The most frequent PTM reaction catalyzed by FIC enzymes is the addition of AMP using ATP as a cofactor, coined AMPylation or adenylylation. Enterococcus faecalis FIC belongs to class III FIC proteins, which are comprised of a single FIC domain and carry an autoinhibitory glutamate in their C-terminal α-helix. We discover that EfFIC has both AMPylation and deAMPylation activities borne by the same active site. Furthermore, the conserved glutamate implements a Ca2+-controlled metal switch that tunes the balance between these activities without conformational change.

We determined crystal structures of unbound, phosphate-bound, AMP-bound, and ATPγS-bound wild-type EfFIC (EfFICWT) and of unbound and sulfate-bound EfFIC carrying a mutation of the catalytic histidine into an alanine (EfFICH111A). All EfFIC monomers resemble closely to each other and to structures of other class III FIC proteins. Notably, the C-terminal α-helix that bears the inhibitory glutamate (E190) shows no tendency for structural flexibility, even in molecules where it is free of crystalline contacts. E190 has the same conformation as in other glutamate-bearing FIC protein structures and is stabilized by a salt bridge with Arg122 and, when present, by interactions with the nucleotide cofactor. EfFIC forms equivalent dimers in all crystal forms, but the arrangement of these dimers in higher-order assemblies varies between crystals. Depending on the crystal forms, EfFIC does not form assemblies larger than the dimers or forms tetramers related to the NmFIC tetramer or forms hexamers comprised of trimers of dimers, making it difficult to establish the functional oligomeric state based on the crystallographic assemblies.

>MHHHHHHMLENKLGIINQLELNRVEERVSKENAKRLYDSGDIDRIEVGTFKGLSYIHNYLFEDIYEFAGKVRSQNISKGNFRFAPVMYLEIALEHIDKMPQRNLDEIVAKYVEMNIAHPFREGNGRATRIWLDLILKKELKRVVDWNLINKEDYLSAMERSPVKDLEIKYLISNALTDKINDREIFMKGIDISYYYEGYTEYNVDEL[4x]>[2x]MNHKVHHHHHHMDVDLGKLFFCGFNDFNEEVKEIIRKYRPTGILIYPGVLSKEYLLMDFMSFLSKEGDFLISSDHEGGQLEVLKYVPSSPGNLAFGKNSPDVTYRYSRVAGKIMEIVGLNMVFAPVLDLLSEESSSVIDIRSYGSDPKIVAEHGARACEGYLEGGVIPCIKHFPGHGKAREDSHLTLPVVDAPFEKLWEEDLLPFRKVLEREKKVTVMTAHVRYSSIDSLPATLSEKIITDVL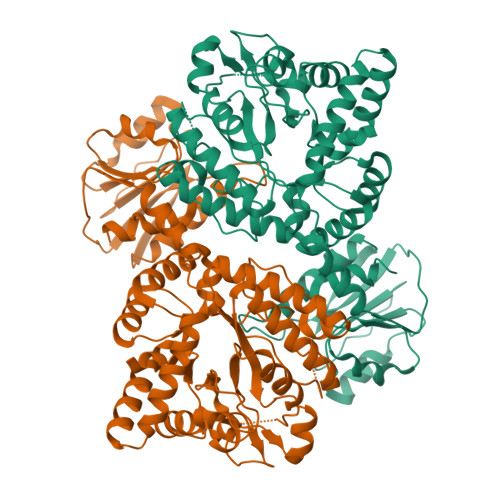REKIGFDGLVISDAMEMSAVSNNFSVEEIVSLFLNAGGNMILLGDYRNLPVYYETLVKLLEDGKVQKDKVERSIRTVEKYLAFAKKNSGVGFLADVSMKAVEFLGFEKIDHTSEVTLLVPSSENLSQADTTGGDYDQIPEIVSRFFEVENVVRYTVEDGPEFVEGDLIFDFVADIPNEKALKAHLSLPAEKTVYFVLRNPFDVRYFEGRKIVVTRSTKPISIYKSLEHFLGRCDS Here, we characterized E. limosum Tub, a tungsten storage protein. Tub has a sub-nanomolar affinity for tungstate and contains a single TOBE domain first characterized in a molybdate storage protein. Crystal structures revealed Tub assembles as a hexamer composed of a trimer of dimers, capable of binding eight tungstate oxyanions at two distinct binding sites located at inter-subunit interfaces. Tub enables E. limosum to accumulate W and then supplies W for two tungstoenzymes needed for conversion of lactate to SCFAs.

A native-gel shift assay of rTub showed that it also bound molybdate and retained its oligomeric nature. Tub demonstrates comparable binding behavior for both tungstate and molybdate in vitro. Similarly, Mo-loaded Tub exhibited the same thermal stability as the W-loaded form and was also resistant to trypsin digestion. While it also binds molybdate in vitro, E. limosum cells preferentially take up W rather than Mo, and its physiological role appears to be to bind tungstate. Whether or not a TOBE protein binds molybdate or tungstate cannot be determined by sequence or structural information alone.

>MKLSARNQLAGKVVSIKEGAVNGIVVLDIGGGNQISSTISMDSIRELGLQVGSDAYAVIKATSVMIGIDDWSHP[6x]> MHHHHHHSSGRENLYFQGSCDFSPGDLVWAKMEGYPWWPCLVYNHPFDGTFIREKGKSVRVHVQFFDDSPTRGWVSKRLLKPYTGSKSKEAQKGGHFYSAKPEILRAMQRADEALN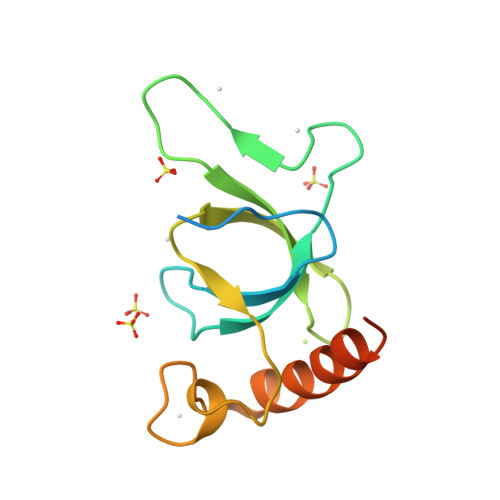KDKIKRLELAVCDE(3S,4R,5R,6S)-azepane-3,4,5,6-tetrol | C6 H13 N O4 | 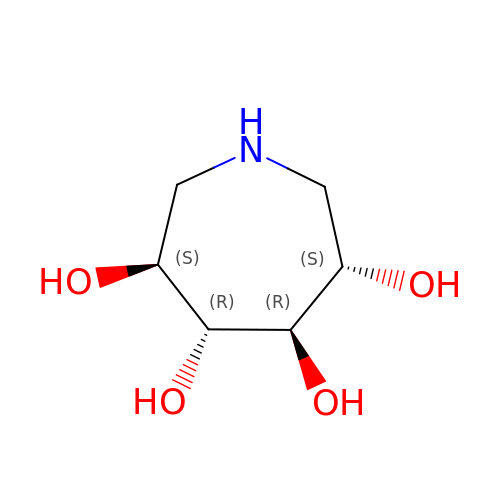MRFFNLOQLBWKPJ-UNTFVMJOSA-N> SMRPALYFCGSIRGGR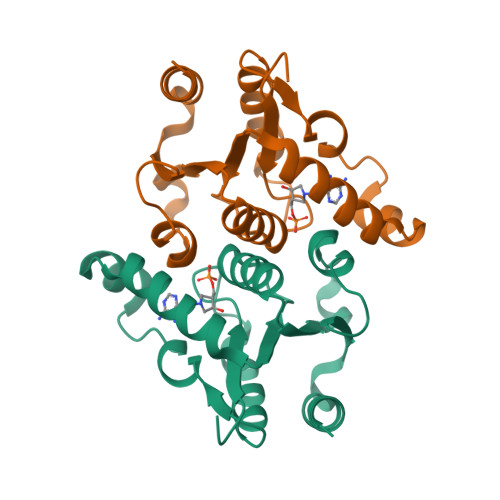EDRTLYERIVSRLRRFGTVLTEHVAAAELGARGEEAAGGDRLIHEQDLEWLQQADVVVAEVTQPSLGVGYELGRAVAFNKRILCLFRPQSGRVLSAMIRGAADGSRFQVWDYEEGEVEALLDRYFEADP>[2x]MSKKNVDPFSDSDSSSEPPSIFSSDNEENSDVDNSVIINDKNTKSDEADIKYMDEDESSDSESESESKKKSKKSKKSKKSKKSVTKKKNNLLVGNRIITEYILIDANNYHFKSWIECFPDCKVNLKLLLFRP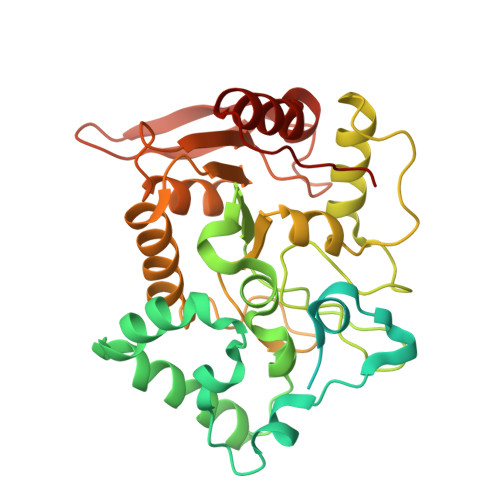EWFDFFKYVESKTYFPQLESKLSSYLEKRQRIVPYPELLFNTMNVLPPGKIKVVILGQDPYPGSCISGVPYAMGCSFSVPLNCPVPKSLANIYTNLIKFNHMRKAPKHGCLASWILQGTFMINSAFTTVLNESGVHARTWESFTADLIDYLTDNYDDLIFVAWGAHAHKLCQRVDPKKHYIITSSHPSPYSVSNTMTSMSYGPNPKKVTYPSFNSVDHFGKINEHLKSRNKKPIFWDL>[2x]ANGVKRWYQKLELPMPPERIFGAHMMLIGGLACLIGTYFFASMTMWNDGYVNLTLRPRLISLGIYDPYDTEQIQRVWLPLIGEFSTSKLPFFGQYPLTMTDFRLFGWGCFHIGLGLWLVYAGAAHYYGARGGATIGEIFWLLPYVPGLKGLCQIKWFTPEGPWYKVGLPWGSFANTPWPILRRTYADALSPHTIYIGLLFFIWGFVLWFVLDKPPVPLQPAQVMTPNGLMPLEQAPFPYGWFDPYLNQVMHPMNTINGETTMCFVWGVLFVALGAYWWYRPPRSINITHLEDTKAVFHVHLTAIGYVSFALAIVGFLALRNHPSYLMLNDMNVIIYGKKIVNPGRMIHNMITFNHVQVGLLYVAAGVFHGGQYLHGLNISGAYKQA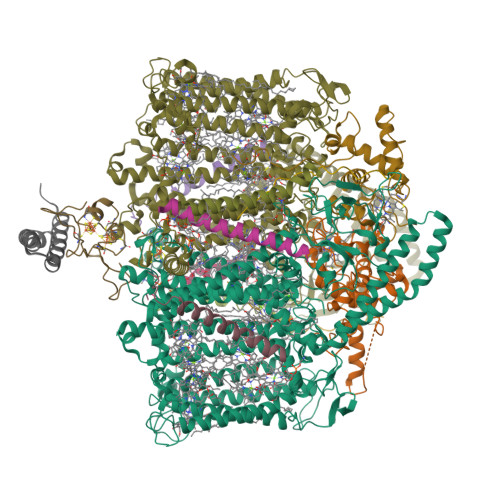RSKFITWFQNPDLQTKIVGTTMFVSFVTVVFGYGMICWNTGAELDLNFGIYQFRSFRAIQMDGEAGNIGYRVFRPKNPWDPTAGGDWVKNPDGTAKLVKARNLQVGDRILNEELGIGSSPTYSFTTIEEINYKPEWGQPKLYAVQWGSWTHFLRKVNPLFWVDKGIWYLQNQKTFEATRKADEAYLAAHLKAVSLLNQIDDAQTEEAKQKAQAELDKFRPELEKAHANMLEWNERLASTPAVLYSNLRDQHRDGEINDAIFFWLMIGGWLFGFIPLLRIAFHNYQSPWYRDFEWRKQSPDFPCIGPVKGGTCGVSIQDQLWFCILFSIKPLSAIAWYLDGGWIATMMARGNEAYYLTHNISHTGGVFLYMWNETTWIWTDNHLTAMLLLGHLIWFVSFALWFKDRGSRAEGGDIQSRWVRLMGKRLGIKTLQEVRFPVSNLATAKLWGTVFFYTGTFVLVFLYFADGFFQNR;> QIYTIIEELCIGCGFCTDECPPKVNAILPRDVEAVLDGGETYWIDQTRCISCSLCFVAGTCPTDAVVFTEGGVSRT;> LLVGGCFVGSRDPNETRYPKAPMPLQNQTSTLKTAEEIRRESVAQNTPGAREAAALRDRVTPLNLQQVNEQDVAGNDPLGSPARVVLDEGEMYRDPVEIYREGRALFQNNCVGCHGHNGCGNVPRSTNFTDPGWQENNSDGGIYSSIYNGKGIGNGGGAMPAYYNQLSPQQIRYLVAYLRAFKGRQCNGLPTLSDVERMVAERQ;> MARTPEEIVKRYKEANIWLRHWKQQIGLAKDEEQREMFTQYYEERVQEIAALEEPYRAALKILNQQESQR;>MTAILLACLFVLGGYAALWGIIKFVVANTKDIAAN[2x];>[2x]MWNVVGQIISVLCFFILTVGTLFGIVYVSHLLSRG;>[2x]DISKVAWAWFGVLLAICLIGAFGNYVPKLFVKMLMFLN;> VMATGCFVGARNASEPRLGSSSIAASRTAPAYLREAQVLYEGSTDGLPKDTPADEIAHYKAMLAELQTRNYAACAGCHQVNGGGNKAINATNFQDAGWQANNSSPGMVTSIVNGKGKVMPAYKDKLTLQQINYLVEYIRRFEKKR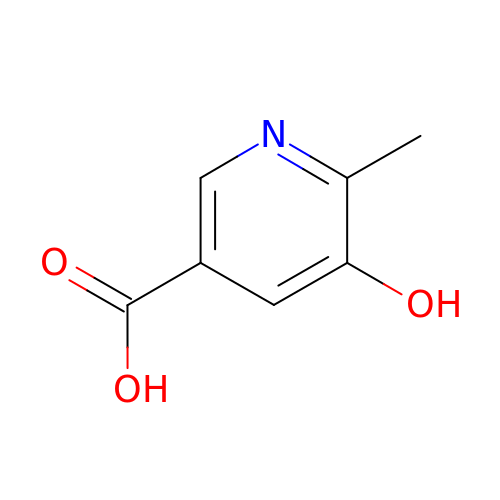5-hydroxy-6-methylpyridine-3-carboxylic acid | C7 H7 N O3 | NYEFWJFPBFRRKU-UHFFFAOYSA-N> MTVSDRELEECIR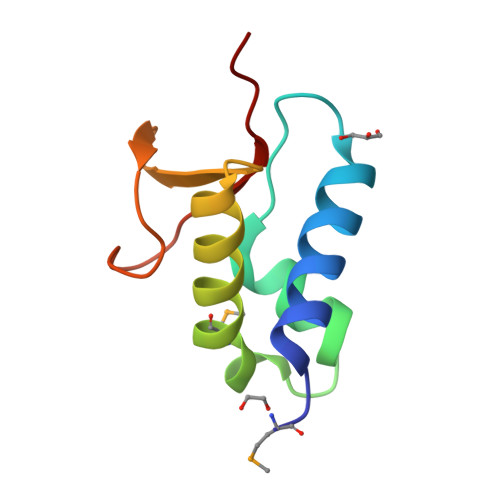ALLDARADSASICPSDVARAVAPDDWRPLMEPVREAAGRLADAGEVEVTQKGAVVDPRSARGPIRIRWTRTD> VGSLNCIVAVSQNMGIGKNGDLPW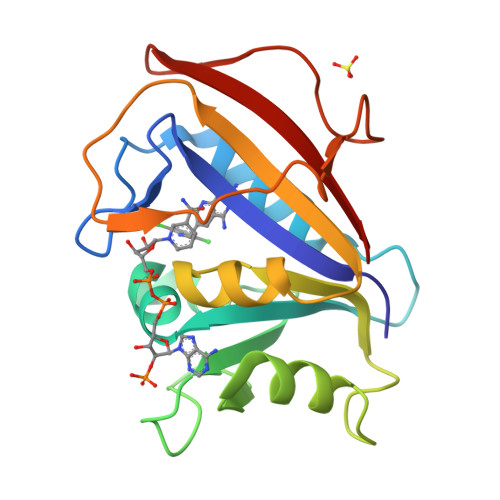PPLRNEFRYFKRMTTTSSVEGKQNLVIMGKKTWFSIPEKNRPLKGRINLVLSRELKEPPQGAHFLSRSLDDALKLTEQPELANKVDMVWIVGGSSVYKEAMNHPGHLKLFVTRIMQDFESDTFFPEIDLEKYKLLPEYPGVLSDVQEEKGIKYKFEVYEKND> LDGVLVPESGILVSVGQDVDSVNDYASALGTIPAGVTNYVGIVNLDGLNSDADAGAGRNNIAELANAYPTSALVVGVSMNGEVDAVASGRYNANIDTLLNTLAGYDRPVYLRWAYEVDGPWNGHSPSGIVTSFQYVHDRIIALGHQAKISLVWQVASYCPTPGGQLDQWWPGSEYVDWVGLSYFAPQDCNWDRVNEAAQFARSKGKPLFLNESTPQRYQVADLTYSADPAKGTNRQSKTSQQLWDEWFAPYFQFMSDNSDIVKGFTYINADWDSQWRWAAPYNEGYWGDSRVQANALIKSNW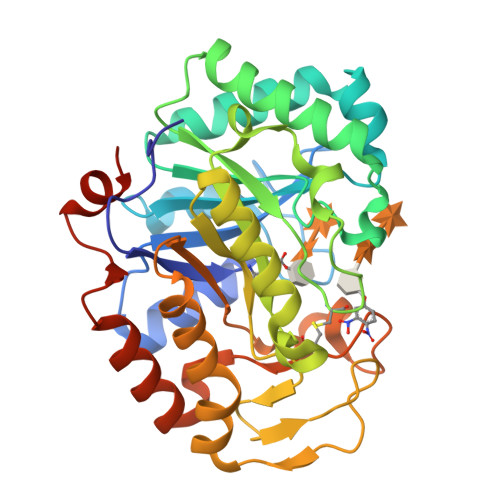QQEIAKGQYINHSETLFETLGYGSTHHHHHH> IINGEDCSPHSQPWQAALVMENELFCSGVLVHPQWVLSAAHCFQNSYTIGLGLHSLEADQEPGSQMVEASLSVRHPEYNRPLLANDLMLIKLDESVSESDTIRSISIASQCPTAGNSCLVSGWGLLANGRMPTVLQCVNVSVVSEEVCSKLYDPLYHPSMFCAGGGQDQKDSCNGDSGGPLICN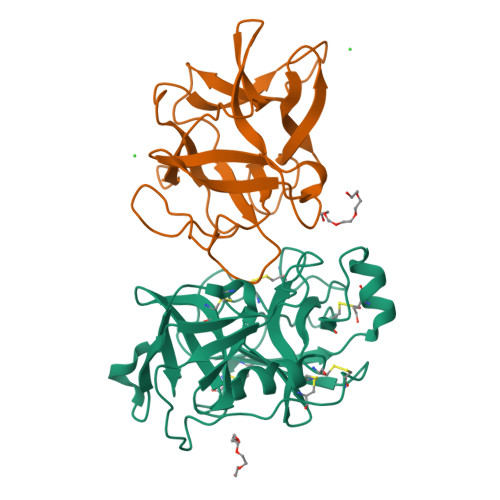GYLQGLVSFGKAPCGQVGVPGVYTNLCKFTEWIEKTVQA;> GSSVVVDTNGQPVSNGADAYYLVPVSHGHAGLALAKIGNEAEPRAVVLDPHHRPGLPVRFESPLFINIIKESYFLNIKFGPSSSDSGVWDVIQQDPIGLAVKVTDTKSLLGPFKVEKEGEGYKIVYYPERGQTGLDIGLVHRNDKYYLAVKDGEPCVFKIRKATDE> MGSERTCCPVNWVEHERSCYWFSRSGKAWADADNYCRLEDAHLVVVTSWEEQKFVQHHIGPVNTWMGLHDQNGPWKWVDGTDYETGFKNWRPEQPDDWYGHGLGGGEDCAHFTDDGRWNDDVCQRPYRWVCETELDKASQEPPLLGSHHHHHH

Herein, bifunctional probes have been developed that target the hepatocyte‐specific asialoglycoprotein receptor (ASGPR), the expression of which decreases during NASH progression. To analyze how the probes, bind to the potential NASH biomarker, X‐ray crystallography and saturation transfer difference nuclear magnetic resonance (STD NMR) spectroscopic methods were used.

The 1.4 Å electron density maps showed unambiguous density not only for the GalNAc moiety, but also for the first 4–7 atoms of the linker. The density for the linker confirmed that the binding site was occupied by our chemical probe, rather than by the free monomeric GalNAc (control experiment) in the mother liquor. In the crystal structure, the 3‐OH and 4‐OH groups of the GalNAc moiety are bound to the calcium ion in ASGPR where the 3‐OH group is in close proximity to the calcium ligands Glu252 and Asn264, while the 4‐OH is very close to the calcium ligands Gln239 and Asp241. In addition, Arg236 makes bidentate hydrogen bonds with the oxygen of the acetyl group and interacts with the oxygen at the 1‐position of GalNAc, where the linker is attached. The nitrogen of the N‐acetyl group interacts with the side chain of Asn264. Finally, the 5‐hydroxymethyl group of GalNAc is stacked onto the indole ring system of Trp243. The linker itself does not appear to interact with ASGPR and is mostly disordered. In comparison, the scaling factors of monomeric GalNAc are significantly lower indicating the lower affinity of the single sugar moiety compared to the triantennary GalNAc groups of the probes GN‐01, GN‐03, and GN‐05. Additionally, the CH2 groups of the aliphatic linker region of these probes show strong, positive STD signals due to binding to ASGPR.>SLKAVIFDLDGVITDTAEYHFLAWKHIAEQIDIPFDRDMNERLKGISREESLESILIFGGAETKYTNAEKQELMHRKNRDYQMLISKLTPEDLLPGIGRLLCQLKNENIKIGLASSSRNAPKILRRLAIIDDFHAIVDPTTLAKGKPDPDIFLTAAAMLDVSPADCAAI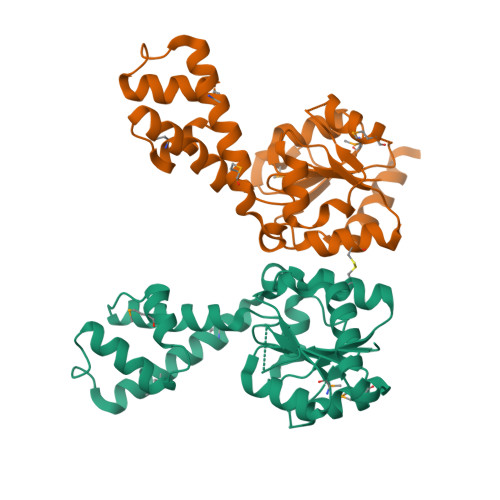EDAEAGISAIKSAGMFAVGVGQGQPMLGADLVVRQTSDLTLELLHEEWEQYRIRESEGHHHHHH[2x]>[2x]MSHHHHHHSMTAKTPLDPALFRPDAISDETRGINDFIIKAFEAVPEWWEIGAATVREARARGEGGFPLPPKSERARTIEIEGKGGHKVPLRIIAPESPKGVYLHIHGGGWVLGACDQQDPMLERIAQNAGLACVSVEYRLAPEHPYPAGPDDCEAAALWLVKNAKKEFGTEVLTIGGESAGGHLSAVTLLRMRDRHGYKGFKGANLVFGAFDMSMSPSQRVFGNERLVLRTVDIQKFGDAFLPNGEDRRDPDISPLYANLHDMPPALFTVGTRDALVDDTLFMHARWIAAGNEAELGVFPGGAHGFVAFP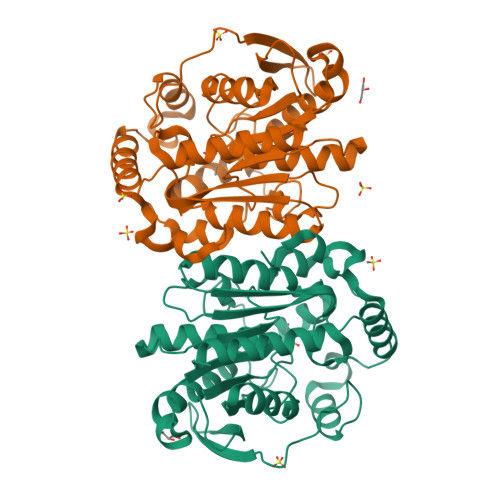GEIARAANAQADAFLRRVTGQ;> MSAKTPLDPALFRPDAISDETRGINDFIIKAFEAVPEWWEIGAATVREARARGEGGFPLPPKSERARTIEIEGKGGHKVPLRIIAPESPKGVYLHIHGGGWVLGACDQQDPMLERIAQNAGLACVSVEYRLAPEHPYPAGPDDCEAAALWLVKNAKKEFGTEVLTIGGESAGGHLSAVTLLRMRDRHGYKGFKGANLVFGAFDMSMSPSQRVFGNERLVLRTVDIQKFGDAFLPNGEDRRDPDISPLYANLHDMPPALFTVGTRDALVDDTLFMHARWIAAGNEAELGVFPGGAHGFVAFPGEIARAANAQADAFLRRVTGQ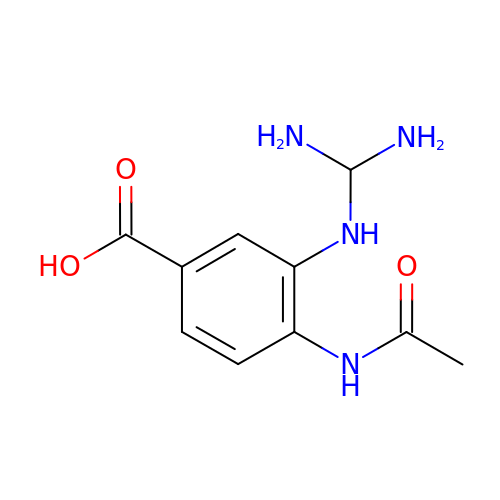4-(ACETYLAMINO)-3-GUANIDINOBENZOIC ACID | C10 H14 N4 O3 | HIXHCUDMJUERSJ-UHFFFAOYSA-N>[17x]MKKITLLLAGSALLLSGCAGVKSSFDCDATTSDTCMTMTKANQLARDKAAKQAGKPAAGGLPSLVNLPATSAVEVPSASRSAVTPPSGTRTVSTTPPVSAGTSAGVNTNTTTSTLTPRPVAGTPVTTTPSSVAYRPVVSVVTPTPSCQNVRCDNPGTVHPQRSRDQIATVWIAPWVDSDNAFHQPGRVSFVVSPADWVLPARVN;>MANVNKVVRRRQVALLIALVLGIGAGGAGTWMVSEMNLKKAPPAKAPKGEPAPDMTGVVNQSFDNKVQRSAIAEAQRLNKETQTEIKKLRTEMGLVSRDLKGSQDRIRELEDQNQLLQTQLEAGKNFDSLSAEPLPGALASQGKPAPAGNVPPPTSFWPAGGGQAPAAPVMTPIQRPGMMDSQEFSLPDTGPKKPRFPWISSGSFVEAIVVEGADANASVTGDKNTAPMQLRLTGKVQMPNDEEFDLTGCFVTL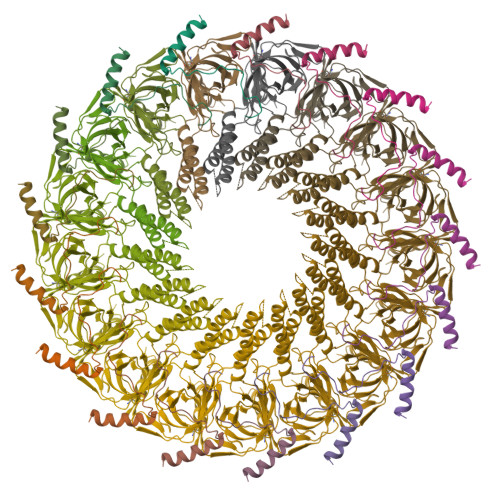EAWGDVSSERAIVRSRSISCKLGDDDIDQKIAGHVSFMGKNGIKGEVVMRNGQILLYAGGAGFLDGIGKGIEKASSTTVGVGATASMSAADIGQAGLGGGVSSAAKTLSDYYIKRAEQYHPVIPIGAGNEVTLVFQDGFQLETLEEARAKAAARKKQNQPSASSTPAAMPGNTPDMLKQLQDFRVGDTVDPATGQVVTQ[17x]> ASVVIRNLSEATHNAIKFRARAAGRSTEAEIRLILDNIAKAQ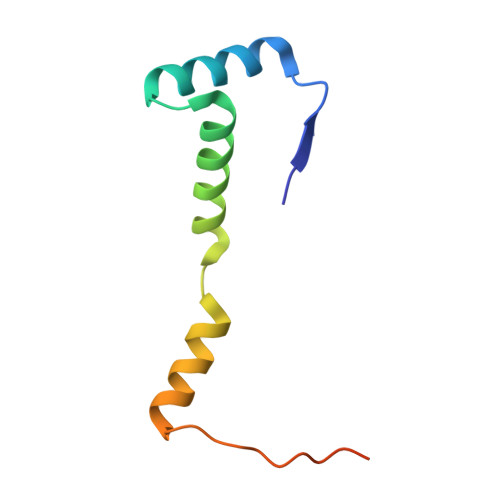QTVRLGSMLASIGQEIGGVELEDVRGRNTDNEVSL> MADVINVSVNLEAFSQAISAIQALRSSVSRVFDCLKDGMRNKETLEGREKAFIAHFQDNLHSVNRDLNELERLSNLVGKPSENHPLHNSGLLSLDPVQDKTPLYSQLLQAYKWSNKLQYHAGLASGLLNQQSLKRSANQMGVSAKRRPKAQPTTLVLPPQYVDDVISRIDRMFPEMSIHLSRPNGTSAMLLVTLGKVLKVIVVMRSLFIDRTIVKGYNENVYTEDGKLDIWSKSNYQVFQKVTDHATTALLHYQL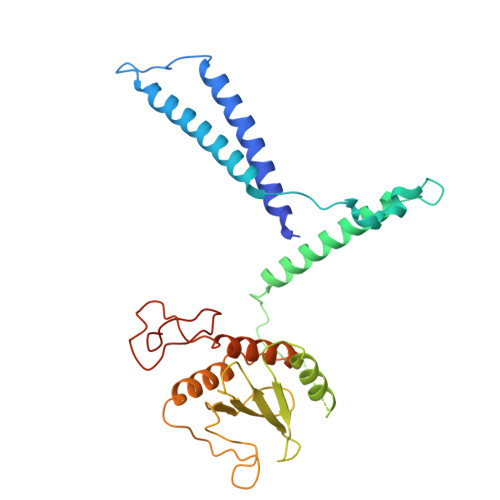PQMPDVVVRSFMTWLRSYIKLFQAPCQRCGKFLQDGLPPTWRDFRTLEAFHDTCRQ>[2x]EAIKWDKAPCRFCGTGCGVLVGTQQGRVVACQGDPDAPVNRGLNCIKGYFLPKIMYGKDRLTQPLLRMKNGKYDKEGEFTPITWDQAFDVMEEKFKTALKEKGPESIGMFGSGQWTIWEGYAASKLFKAGFRSNNIDPNARHCMASAVVGFMRTFGMDEPMGCYDDIEQADAFVLWGANMAEMHPILWSRITNRRLSNQNVTVAVLSTYQHRSFELADNGIIFTPQSDLVILNYIANYIIQNNAINQDFFSKHVNLRKGATDIGYGLRPTHPLEKAAKNPGSDASEPMSFEDYKAFVAEYTLEKTAE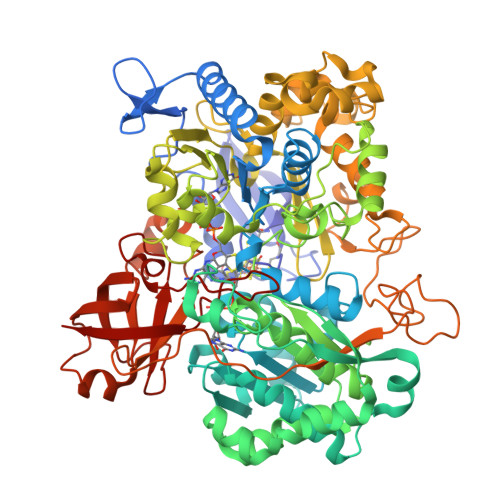MTGVPKDQLEQLAQLYADPNKKVISYWTMGFNQHTRGVWANNLVYNLHLLTGKISQPGCGPFSLTGQPSACGTAREVGTFAHRLPADMVVTNEKHRDICEKKWNIPSGTIPAKIGLHAVAQDRALKDGKLNVYWTMCTNNMQAGPNINEERMPGWRDPRNFIIVSDPYPTVSALAADLILPTAMWVEKEGAYGNAERRTQFWRQQVQAPGEAKSDLWQLVQFSRRFKTEEVWPEDLLAKKPELRGKTLYEVLYATPEVSKFPVSELAEDQLNDESRELGFYLQKGLFEEYAWFGRGHGHDLAPFDDYHKARGLRWPVVNGKETQWRYSEGNDPYVKAGEGYKFYGKPDGKAVIFALPFEPAAEAPDEEYDLWLSTGRVLEHWHTGSMTRRVPELHRAFPEAVLFIHPLDAKARDLRRGDKVKVVSRRGEVISIVETRGRNRPPQGLVYMPFFDAAQLVNKLTLDATDPLSKETDFKKCAVKLEKV>LQPLPPTAFTPNGTYLQHLARDPTSGTLYLGATNFLFQLSPGLQLEATVSTGPVLDSRDCLPPVMPDECPQAQPTNNPNQLLLVSPGALVVCGSVHQGVCEQRRLGQLEQLLLRPERPGDTQYVAANDPAVSTVGLVAQGLAGEPLLFVGRGYTSRGVGGGIPPITTRALWPPDPQAAFSYEETAKLAVGRLSEYSHHFVSAFARGASAYFLFLRRDLQAQSRAFRAYVSRVCLRDQHYYSYVELPLACEGGRYGLIQAAAVATSREVAHGEVLFAAFSSAAPPTVGRPPSAAAGASGASALCAFPLDEVDRLANRTRDACYTREGRAEDGTEVAYIEYDVNSDCAQLPVDTLDAYPCGSDHTPSPMASRVPLEATPILEWPGIQLTAVAVTMEDGHTIAFLGDSQGQLHRVYLGPGSDGHPYSTQSIQQGSAVSRDLTFDGTFEHLYVMTQSTLLKVPVASCAQHLDCASCLAHRDPYCGWCVLLGRCSRRSECSRGQGPEQWLWSFQPELGCLQKHHHHHH[2x]

Plexin-B1 is a receptor for the cell surface semaphorin, Sema4D. pmcThe plexins are a family of cell surface single transmembrane domain receptors for cell surface and soluble semaphorins. The extracellular domains of plexins consist of three domain types: the IPT domain (immunoglobulin domain shared by plexins and transcription factors), the PSI domain (lexins, semaphorins, and integrins), and the sema domain. The sema domain is a seven-bladed β-propeller domain, with a large insert which gives the sema domain a distinctive, asymmetrical shape.

To further understand the mechanism of the VHHs inhibition of Sema4D binding to Plexin-B1, the structure of human Plexin-B1 (20–535) was solved by X-ray crystallography to a resolution of 2.69 Å, with the asymmetric unit containing two copies of hPlexin-B1. Several cadmium ions were found in the crystal structure, some of which support the crystal packing observed. Initial Cα RMSD comparisons of the two chains found in the apo human Plexin-B1 structure revealed that the PSI domain (480–535) undergoes significant loop movements within the crystal form, as do several loops in the sema domain. Contrary to what has been reported for Plexin-A2 (18), our analysis revealed significant loop movements in Plexin-B1 induced by Sema4D binding, which extend beyond the binding interface of Sema4D. The largest movements seen are up to 15.2 Å in the position of the A5-B5 loop. In the apo structure, this loop is folded over and interacts with the cleft between blades 5 and 6 of the sema domain. This region in the structure is the site to which the allosteric inhibitory peptide PB1m6 peptide binds to which was previously thought to be a preformed cleft in the sema domain. Regions of increased RMSD also identify that conformational changes are seen in several loops on both faces of the sema domain, such as the A3-B3 loop, the B3-C3 loop, B4-C4 loop, C4-D4 loop, B5-C5 loop, and the C6-D6 loop. The C6-D6 loop is adjacent to the cleft formed by the motion of the A5-B5 loop in the Sema4D bound structure and is further retracted from this region in the apo structure, presumably to allow space for the insertion of the A5-B5 loop in the apo structure reported here. The work presented here questions this paradigm by showing that the sema domain of Plexin-B1 undergoes significant structural rearrangement upon semaphorin binding.>MGSDKIHHHHHHENLYFQGMARYINITLEKRGVTCKALLLDDVAPRTSKAVWDALPQSS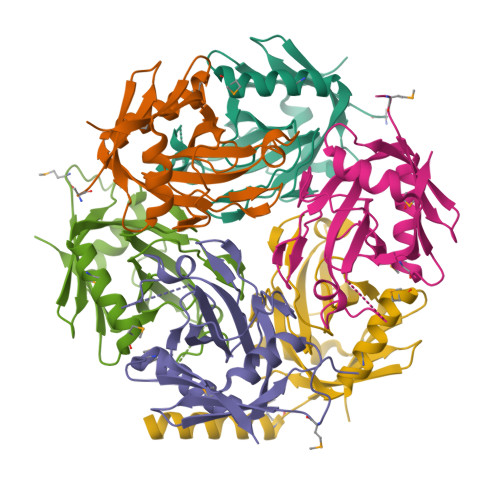QVFHGKYARNEIYNLVPAFAPKEPGAENTTVTPIPGDVCYFTFTSNDLKTPSHGYEADSGTDEVQTIVDLAVFYGRNNLLLNGDTGWVPGNVFATIVEGLDEMAAACQDIWMGGARDETLTFSRAEDTA[6x]>MGEQPIFTTRAHVFQIDPSTKKNWVPASKQAVTVSYFYDVTRNSYRIISVDGAKVIINSTITPNMTFTKTSQKFGQWADSRANTVFGLGFSSELQLTKFAEKFQEVRE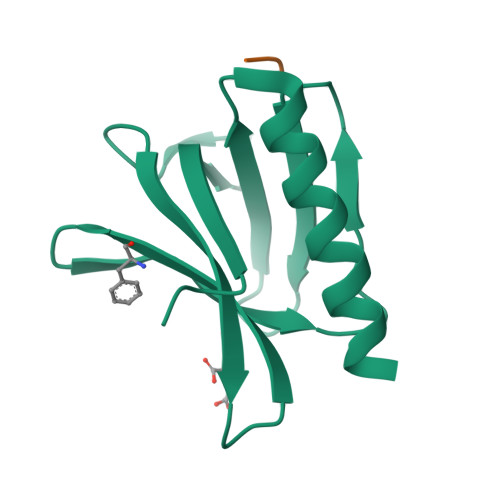AAR[4x];> FAF>MADVTGIALGMIETRGLVPAIEAADAMTKAAEVRLVGRQFVGGGYVTVLVRGETGAVNAAVRAGADACERVGDGLVAAHIIARVHSEVENILPKAPQA[15x];> MKIMQVEKTLVSTNRIADMGHKPLLVVWEKPGAPRQVAVDAIGCIPGDWVLCVGSSAAREAAGSKSYPSDLTIIGIIDQWNGE;>[2x]MPFCTSTPEPEAQSTEQSLTCEGQIISGTSVDASDLVTGNEIGEQQLISGDAYVGAQQTGCLPTSPRFNQTGNVQSMGFKNTNQPEQNFAPGEVMPTDFSIQTPARSAQNRITGNDIAPSGRITGPGMLATGLITGTPEFRHAARELVGSPQPMAMAMANRNKAAQAPVVQPEVVATQEKPELVCAPRSDQMDRVSGEGKERCHITGDDWSVNKHITGTAGQWASGRNPSMRGNARVVETSAFANRNVPKPEKPGSKITGSSGNDTQGSLITYSGGARG

Among diverse BMCs, carboxysomes are specific CO2-fixing BMCs found in all cyanobacteria and many proteobacteria. The carboxysome uses a polyhedral protein shell to encapsulate the key CO2 fixation enzymes, ribulose-1,5-bisphosphate carboxylase/oxygenase (Rubisco) and carbonic anhydrase (CA). Carboxysome shells are typically composed of three groups of structural components that form hexamers, pentamers, and trimers. Here, we generated recombinant α-carboxysome shells of Halothiobacillus neapolitanus by expressing all the shell proteins (involving three CsoS1 hexameric proteins and two CsoS4 pentameric proteins), together with the C-terminal domain of CsoS2 (CsoS2-C) that mediates shell assembly.

The cryo-EM structures of T = 9, T = 9 Q = 12, T = 13, T = 16, and T = 19 shell assemblies were determined at 2.3-, 2.99-, 2.93-, 2.75-, and 3.04-Å resolution, respectively. In the T = 16 shell, the identified CsoS2-C regions encompass almost identical F1 to F5 fragments as those of the T = 19 shell. Intriguingly, the smaller T = 9 shells involved only one conformation of CsoS2-C, whereas the second conformation of CsoS2 appeared in the larger T = 13, T = 16, and T = 19 shells. To visualize the existence of CsoS1A/B heterohexamers and prevent symmetry-caused biases in the process of differentiating CsoS1A and CsoS1B in the shells, we also analyzed the structures without introducing additional symmetries. Fortunately, the density maps for the T = 9 (C1) and T = 16 (C1) shells were retained at good resolution. For the T = 16 (C1) shell map, additional densities consistent with the CsoS1B C-terminal helix were observed at the central and terminal regions of the CsoS1 hexamer. Although building the structural model was challenging at this density, this result confirms that CsoS1A and CsoS1B can form heterohexamers during shell assembly. Collectively, these results imply that there is a correlation between the size/structure of the shell and the incorporation of CsoS1A/B heterohexamers and that CsoS1B is probably highly abundant in the larger shells.N-(tert-butoxycarbonyl)-3-methyl-L-valyl-(4R)-4-[(7-chloro-4-methoxyisoquinolin-1-yl)oxy]-N-[(1R,2R)-1-[(cyclopropylsulfonyl)carbamoyl]-2-(difluoromethyl)cyclopropyl]-L-prolinamide 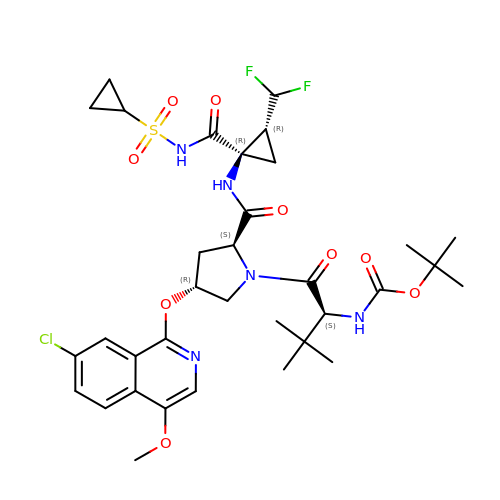| C34 H44 Cl F2 N5 O9 S | PSVSXONHXYMVQH-GGFAASIMSA-N2-[4-[(1~{S})-1-[[4,5-bis(chloranyl)-1,6-dimethyl-indol-2-yl]carbonylamino]-2-oxidanyl-ethyl]phenyl]sulfonylethanoic acid | C21 H20 Cl2 N2 O6 S | 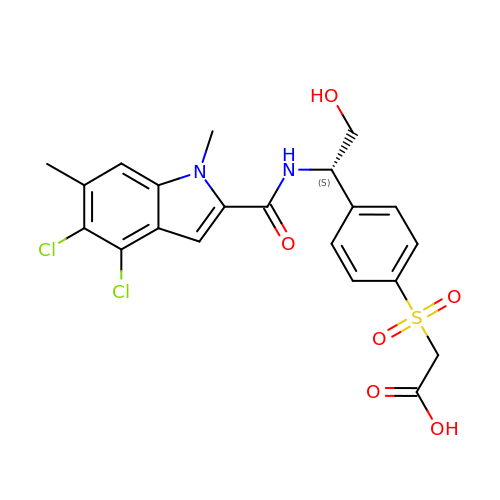CJEJFFCPVBZSIE-OAHLLOKOSA-N>GSHMASSESTEEKPDTDLADKYASGNSEISGQELRGLRDAIGDDASPEDILALVQEKIKDPALQSTALDYLVQTTPPSQGKLKEALIQARNTHTEQFGRTAIGAKNILFASQEYADQLNVSPSGLRSLYLEVTGDTHTCDQLLSMLQDRYTYQDMAIVSSFLMKGMATGLKRQGPYVPSAQLQVLMTETRNLQAVLTSYDYFESRVPILLDSLKAEGIQTPSDLNFVKVAESYHKIINDKFPTASKVEREVRNLIG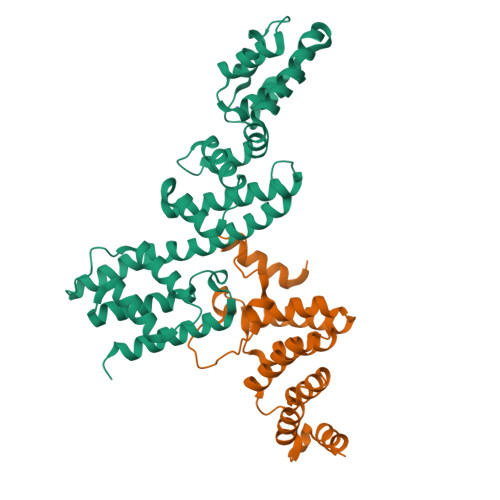DDVDSVTGVLNLFFSALRQTSSRLFSSADKRQQLGAMIANALDAVNINNEDYPKASDFPKPYPWS[2x];>GSHMASMSHLNYLLEKIAASSKEDFPFPDDLESYLEGYVPDKNIALDTYQKIFKISSEDLEKVYKEGYHAYLDKDYAKSITVFRWLVFFNPFVSKFWFSLGASLHMSEQYSQALHAYGVTAVLRDKDPYPHYYAYICYTLTNEHEEAEKALEMAWVRAQHKPLYNELKEEILDIRKHK[2x]> SSTNV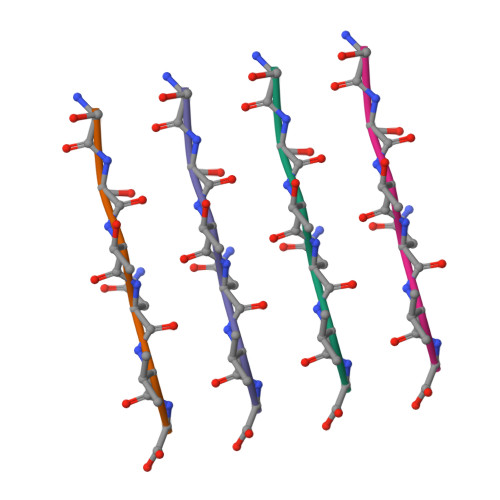G> SMTTNVGDSTLADLLDHSCTSGSGSGLPFLVQRTVAREITLLECVGKGRYGEVWRGSWQGENVAVKIFSSRDEKSWFRETELYNTVMLRHENILGFIASDMTSRHSSTQLWLITHYHEMGSLYDYLQLTTLDTVSCLRIVLSIASGLAHLHIEIFGTQGKPAIAHRDLKSKNILVKKNGQCCIADLGLAVMHSQSTNQLDVGNNPRVGTKRYMAPEVLDETIQVDCFDSYKRVDIWAFGLVLWEVARRMVSNGIVEDYKPPFYDVVPNDPSFEDMRKVVCVDQQRPNIP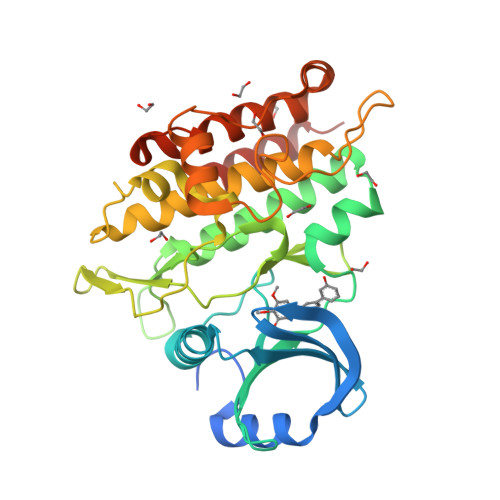NRWFSDPTLTSLAKLMKECWYQNPSARLTALRIKKTLTKIDNSLDKLKTDC>[2x]MHHHHHHTSKIEQPRWASKDSAAGAASTPDEKIVLEFVDALTSNDAAKLIEYFAEDTMYQNMPLPPAYGRDAVEQTLAGLFTVVSVDAV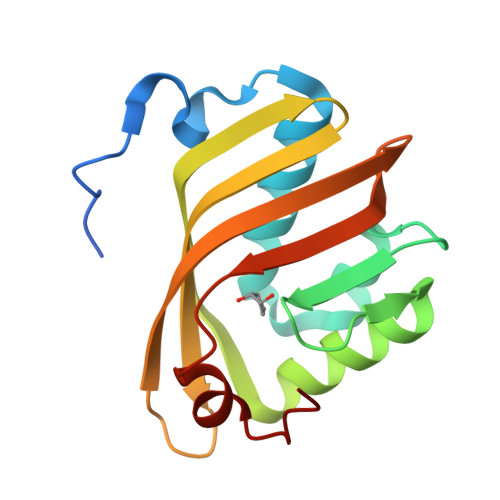ETFHIGSSNGLVYTERVDVLRALPTGKSYNFSILGVFQLTEGKITGWRDYFDLREFEEAVDLPLRG>MVKSFLMLGQSNMAGRGFINEVPMIYNERIQMLRNGRWQMMTEPINYDR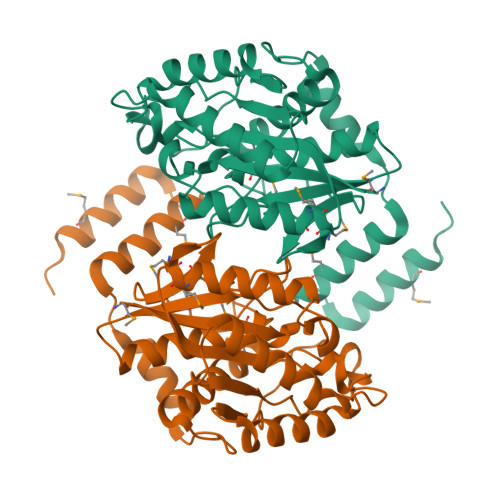PVSGISLAGSFADAWSQKNQEDIIGLIPCAEGGSSIDEWALDGVLFRHALTEAKFAMESSELTGILWHQGESDSLNGNYKVYYKKLLLIIEALRKELNVPDIPIIIGGLGDFLGKERFGKGCTEYNFINKELQKFAFEQDNCYFVTASGLTCNPDGIHIDAISQRKFGLRYFEAFFNRKHVLEPLINENELLNLNYARTHTKAEKIYIKSMDFALGKISYDEFTSELMKINNDLEHHHHHH[6x]>MGSDKIHHHHHHMSEPVIKSLLDTDMYKITMHAAVFTNFPDVTVTYKYTNRSSQLTFNKEAINWLKEQFSYLGNLRFTEEEIEYLKQEIPYLPSAYIKYISSSNYKLHPEEQISFTSEEIEGKPTHYKLKILVSGSWKDTILYEIPLLSLISEAYFKFVDIDWDYENQLEQAEKKAETLFDNGIRFSEFGTRRRRSLKAQDLIMQGIMKAVNGNPDRNKSLLLGTSNILFAKKYGVKPIGTVAHEWVMGVASISEDYLHANKNAMDCWINTFGAKNAGLALTDTFGTDDFLKSFRPPYSDAYVGVR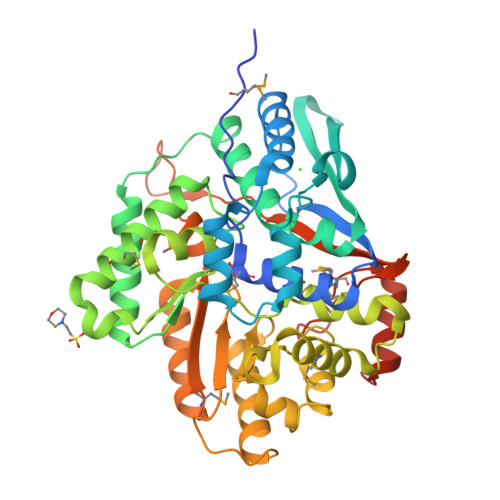QDSGDPVEYTKKISHHYHDVLKLPKFSKIICYSDSLNVEKAITYSHAAKENGMLATFGIGTNFTNDFRKKSEPQVKSEPLNIVIKLLEVNGNHAIKISDNLGKNMGDPATVKRVKEELGYTERSWSGDNEAHRWT[4x]> MSGPERITLAMTGASGAQYGLRLLDCLVQEEREVHFLISKAAQLVMATETDVALPAKPQAMQAFLTEYCGAAAGQIRVFGQNDWMAPPASGSSAPNAMVICPCSTGTLSAVATGACNNLIERAADVALKERRPLVLVPREAPFSSIHLENMLKLSNLGAVILPAAPGFYHQPQSVEDLVDFVVARILNT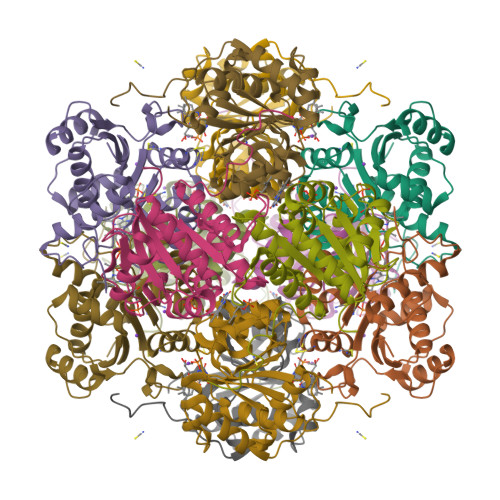LGIPQDMLPRWGEQHLVSDE>PREVLTGGHSVSAPQENRIYVMDSVFMHLTESRVHVYDYTNGKFLGMVPTAFNGHVQVSNDGKKIYTMTTYHERITRGKRSDVVEVWDADKLTFEKEISLPPKRVQGLNYDGLFRQTTDGKFIVLQNASPATSIGIVDVAKGDYVEDVTAAAGCWSVIPQPNRPRSFMTICGDGGLLTINLGEDGKVASQSRSKQMFSVKDDPIFIAPALDKDKAHFVSYYGNVYSADFSGDEVKVDGPWSLLNDEDKAKNWVPGGYNLVGLHRASGRMYVFMHPDGKEGTHKFPAAEIWVMDTKTKQRVARIPGRDALSMTIDQQRNLMLTLDGGNVNVYDISQPEPKLLRTIEGAAEASLQVQFHPVGGT[2x];>HISLNPDLANEDEVNSCDYWRHCAVDGFLCSCC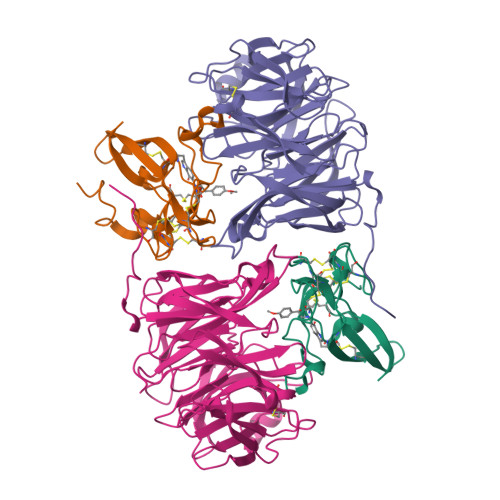GGTTTTCPPGSTPSPISWIGTCHNPHDGKDYLISYHDCCGKTACGRCQCNTQTRERPGYEFFLHNDVNWCMANENSTFHCTTSVLVGLA[2x]>MRTIIALETHDVRFPTSRELDGSDAMNPDPDYSAAYVVLRTDGAEDLAGYGLVFTIGRGNDVQTAAVAALAEHVVGLSVDKVIADLGAFARRLTNDSQLRWLGPEKGVMHMAIGAVINAAWDLAARAANKPLWRFIAELTPEQLVDTIDFRYLSDALTRDEALAILRDAQPQRAARTATLIEQGYPAYTTSPGWLGYSDEKLVRLAKEAVADGFRTIKLKVGANVQDDIRRCRLARAAIGPDIAMAVDANQRWDVGPAIDWMRQLAEFDIAWIEEPTSPDDVLGHAAIRQGITPVPVSTGEHTQNRVVFKQLLQAGAVDLIQIDAARVGGVNENLAILLLAAKFGVRVFPHAGGVGLCELVQHLAMADFVAITGK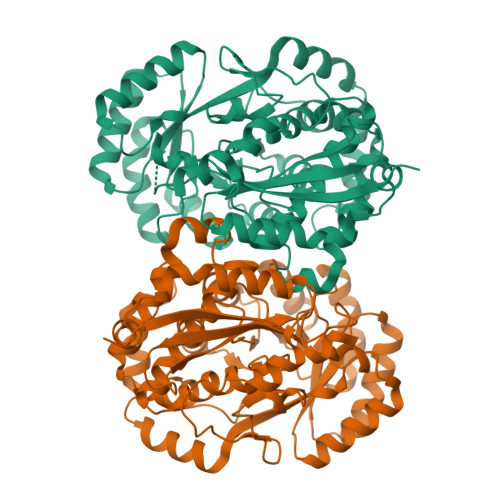MEDRAIEFVDHLHQHFLDPVRIQHGRYLAPEVPGFSAEMHPASIAEFSYPDGRFWVEDLAA[4x]>[6x]GAMGSGIQMKEEASEHGGSADETQELSPVSDSSDEMPNNAKRRRRSQSMIANKRIHQAFQEDEGDEDWEEEEHKPKAKRRYNTRSNESFSEGDDEPFEVSESSALEDELSDSEDSFIRSVRSKPKYKPGTRRSTRLRNRRSQDEEESEEEHRPILRERTSRINYSVPLAFPPVDEMDGDPSSQVNQSRSRKTHSELAITKLLRQQVSSFMPYIDSSGSESESDNTRIKKSSAKTIKALTDPANSGGPPDFGRIREKSDLADSDPLGVDSSLSFESVGGLDNYINQLKEMVMLPLLYPEIFQRFNMQPPRGVLFHGPPGTGKTLMARALAAACSSENKKVSFYMRKGADCLSKWVGEAERQLRLLFEEAKSTQPSIIFFDEIDGLAPVRSSKQEQIHASIVSTLLALMDGMESRGQVIIIGATNRPDAVDPALRRPGRFDREFYFPLPDRDARKKIIEIHTRNWDPPVPEWLCSMLAEKSKGYGGADLRALCTEAALNSIKRTYPQLYRSTKRLQIDPKTIKVKVKDFVMSMKRMIPSSERSSISPSKPLSPELKPLLNEAFQDIEKTLQKLMPVASKLNPLEEVMYDDPKENDFEYQQRLETFETLRIYKPRFLICGRKGLGQTALGPAILQQYEGVHVQSFDMSTLLQDSTQSIETSIIHLFLEVRRHTPSIIYIPDIDNWLNVLPLTAITTFSSMLERLDFSDQILFLALSSSPLSELHPQLREWFSSKQSVYSLQYPTRDSIIAFFQPILELIKASPTELPGGIPRKRRVLPELPLAPDPPPFTSQKITLKQTKQADMRLLNKLKIKLNALLGSLRARYRKFKKPLIDFNDIYCVDPETGHSYRSREECHYEFVDDVVKQIGSDQKFSMMSLEEIEKRTWDNCYCTPKQFVHDIKLILRDALQLEDSETIKRAQEMYANVLLGVEDMEDDQFSQRCERMALREAERRKLRHGKLQKHLDETKADMQFTSEKPSVDESITEVDDAIKDGPPVLAETLTNSLMEDVGPENVDMDIEDNEIFTNQSTMSVPSMLVENEESPKPDEYIDQKDKVQSPLLNGKSPVGVPSEAALRVSTDVSTNISSNGRADIPVDTLITSPADVPNNAPTDAHNITSADGHIENIEQEVVFPDLVFDEDRLTPLKQLLIDSTTGFTVDQLLHLHSFLYQIIWNTKSEWNRNSVVDECERAVKEFMINALQ

ATAD2 (also termed ANCCA) is a histone chaperone that has been implicated in nucleosome density regulation by histone H3–H4 loading or removal. Although histone chaperones responsible for nucleosome assembly and disassembly usually do not contain ATPase domains, ATAD2 is unique because it is the only known AAA+ ATPase histone chaperone. Here, we demonstrate ATP-dependent histone H3–H4 deposition onto DNA by Abo1, the fission yeast ortholog of ATAD2, using an in vitro single-molecule imaging technique, the DNA curtain. We solve the cryo-EM structures of Abo1 in three different nucleotide states (apo, ADP, and ATP), revealing a major reorganization of the AAA+ domains from an open spiral to a closed ring—a structural change that can also be recapitulated in real time by high-speed atomic force microscopy (HS-AFM).

In addition, we determined two cryo-EM structures in apo-states. One structure was determined to 4.3 Å resolution, which is similar in resolution to ADP-Abo1. The other structure that showed clear features of the bromodomain was determined to 6.9 Å resolution from data collected using a Volta phase plate. Therefore, we used the 4.3 Å resolution structure of apo-Abo1 for comparing with ATP- or ADP- bound states, and referred to the lower resolution structure of apo-Abo1 for describing the bromodomain. Especially in the low resolution cryo-EM structure of the apo-state, six lobes of density that match the expected dimensions of a bromodomain were arranged in a hexameric ring around a central lobe of density. On the outer face of the bromodomain ring, characteristic helical densities that run diagonal to the central ring axis could be observed. In addition, we also observed an extra density at the center of the bromodomains, although it is unclear whether this is part of Abo1 or a bound substrate. In most asymmetric states, only one blade disappeared from the field of view, but there were also rare transient cases where two blades of the ring disappeared simultaneously. These HS-AFM results were highly consistent with our cryo-EM structures that show a closed symmetric ring for apo- and ADP states and an open spiral in the ATP-state. The “hole” is formed by the AAA1 HBD, AAA2 HBD, and a linker that proceeds the AAA2 HBD. This unique addition, which we name the “linker arm”, stabilizes the hexameric conformation and explains how Abo1, in contrast to other AAA+ ATPases, can exist as a stable hexamer even in the absence of nucleotide.> GLVPRGSHMMEILRGSPALSAFRINKLLARFQAANLQVHNIYAEYVHFADLNAPLNDSEQAQLTRLLQYGPALSSHTPAGKLLLVTPRPGTISPWSSKATDIAHNCGLQQVDRLERGVAYYIEASTLTAEQWRQVAAELHDRMMETVFSSLTDAEKLFIHHQPAPVSSVDLLGEGRQALIDANLRLGLALAEDEIDYLQEAFTKLGRNPNDIELYMFAQANSEHCRHKIFNADWIIDGKPQPKSLFKMIKNTFETTPDYVLSAYKDNAAVMEGSAVGRYFADHNTGRYDFHQEPAHILMKVETHNHPTAISPWPGAATGSGGEIRDEGATGRGAKPKAGLVGFSVSNLRIPGFEQPWEEDFGKPERIVTALDIMTEGPLGGAAFNNEFGRPALTGYFRTYEEKVNSHNGEELRGYHKPIMLAGGIGNIRADHVQKGEIVVGAKLIVLGGPAMNIGLGGGAASSMASGQSDADLDFASVQRDNPEMERRCQEVIDRCWQLGDANPILFIHDVGAGGLSNAMPELVSDGGRGGKFELRDILSDEPGMSPLEIWCNESQERYVLAVAADQLPLFDELCKRERAPYAVIGDATEEQHLSLHDNHFDNQPIDLPLDVLLGKTPKMTRDVQTLKAKGDALNRADITIADAVKRVLHLPTVAEKTFLVTIGDRTVTGMVARDQMVGPWQVPVADCAVTTASLDSYYGEAMSIGERAPVALLDFAASARLAVGEALTNIAATQIGDIKRIKLSANWMAAAGHPGEDAGLYDAVKAVGEELCPQLGLTIPVGKDSMSMKTRWQEGNEQREMTSPLSLVISAFARVEDVRHTLTPQLSTEDNALLLIDLGKGHNALGATALAQVYRQLGDKPADVRDVAQLKGFYDAMQALVAARKLLAWHDRSDGGLLVTLAEMAFAGHCGVQVDIAALGDDHLAALFNEELGGVIQVRAEDRDAVEALLAQYGLADCVHYLGQALAGDRFVITANDQTVFSESRTTLRVWWAETTWQMQRLRDNPQCADQEHEAKANDTDPGLNVKLSFDINEDIAAPYIATGARPKVAVLREQGVNSHVEMAAAFHRAGFDAIDVHMSDLLGGRIGLGNFHALVACGGFSYGDVLGAGEGWAKSILFNHRVRDEFETFFHRPQTLALGVCNGCQMMSNLRELIPGSELWPRFVRNHSDRFEARFSLVEVTQSPSLLLQGMVGSQMPIAVSHGEGRVEVRDDAHLAALESKGLVALRYVDNFGKVTETYPANPNGSPNGITAVTTENGRVTIMMPHPEAVFRTVANSWHPENWGEDSPWMRIFRNARKQLG

FGAR-AT encoded by the purL gene is a multidomain bi-functional enzyme that catalyzes the fourth step of the purine biosynthesis pathway. The FGAR-AT protein from Salmonella typhimurium (StPurL) has 1295 amino acid residues and is a single chain protein with three major domains. The C-terminal glutaminase domain produces an ammonia molecule that is consumed at the coupled active site present in the formylglycinamidine ribonucleotide (FGAM) synthetase domain where nitrogen is incorporated into an FGAR molecule converting it into FGAM. While the FGAM synthetase domain and glutaminase domain carry out the two enzymatic reactions within this bi-functional enzyme, the function of the N-terminal domain is not clearly understood.

Data sets of the xenon bound structure of StPurL were collected and refined using both native and a mutant version of StPurL R1263A. This mutant was analyzed and was found to be structurally identical to the xenon data set of the native protein (2.65 Å) and diffracted to a higher resolution of 2.18 Å and therefore, used for further analysis. Five xenon atoms were located using mFo-DFc map and confirmed using an anomalous difference fourier map. However, only three out of them were buried in the core. The other two xenon sites occupied shallow hydrophobic patches on the surface of the protein formed by crystal packing contacts, therefore were deemed functionally unimportant. The first xenon site (Xe1) was found nested in the hydrophobic barrel characteristic of type I glutaminases in the ammonia production domain that constitutes 24% of the total protein. The second xenon atom (Xe2) was located in the FGAM synthetase domain, trapped at the edge of the hydrophobic barrel formed between the two gene duplicated halves of this domain. The third xenon atom (Xe3) was located at the interface of the three helix N-terminal linker domain and the central FGAM synthetase domain. However, X-ray crystallographic studies revealed that none of the three internal xenon atoms were trapped in either of the proposed ammonia channels within the protein instead they were bound to select hydrophobic spaces within. Therefore, it is likely that the compact fold of the protein results in very few surface exposed hydrophobic patches leading to only three internal xenon atoms being structurally trapped.>PQFSLWKRPVVTAYIEGQPVEVLLDTGADDSIVAGIELGNNYSPKIVGGIGGFINTKEYKNVEIEVLNKKVRA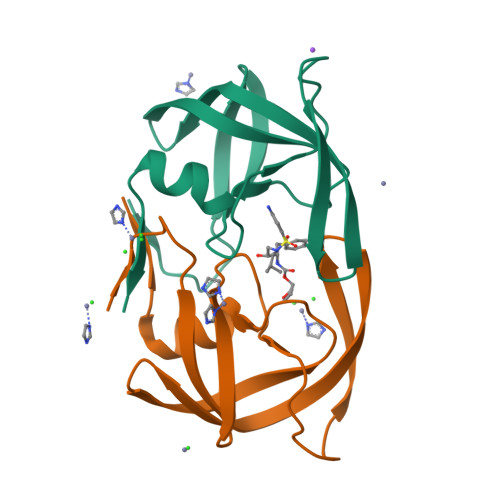TIMTGDTPINIFGRNILTALGMSLNL[2x]[2-amino-3-(4-bromobenzoyl)phenyl]acetic acid 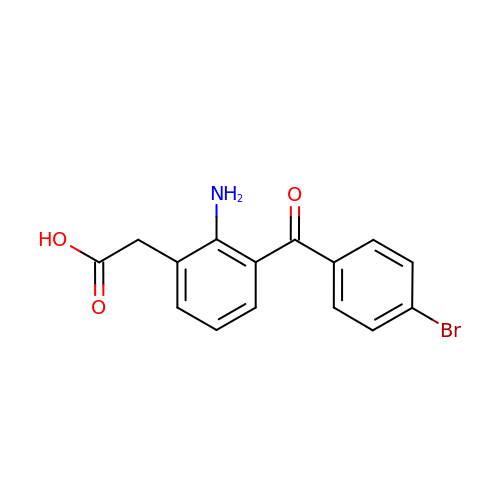| C15 H12 Br N O3 | ZBPLOVFIXSTCRZ-UHFFFAOYSA-N>[4x]DLHEILHEAVPLDANEREILELKE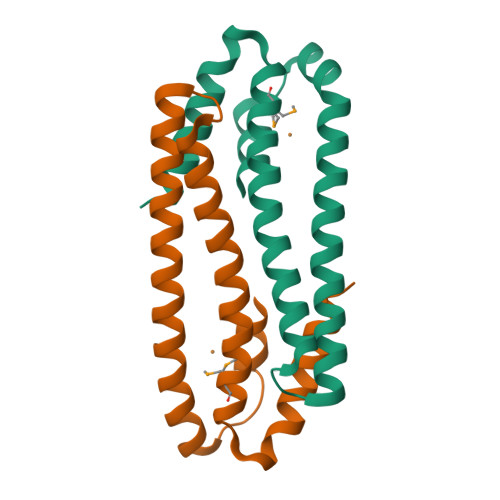DAFAQRRREIETRLRAANGKLADAIAKNPAWSPEVEAATQEVERAAGDLQRATLVHVFEMRAGLKPEHRPAYDRVLIDALRRGSQ> MGSSHHHHHHSQDPNSMTTLTRQDLNFGQVVADVLCEFLEVAVHLILYVREVYPVGIFQKR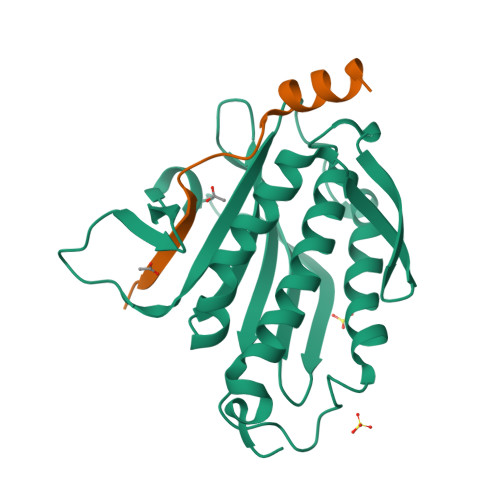KKYNVPVQMSCHPELNQYIQDTLHCVKPLLEKNDVEKVVVVILDKEHRPVEKFVFEITQPPLLSISSDSLLSHVEQLLAAFILKISVCDAVLDHNPPGCTFTVLVHTREAATRNMEKIQVIKDFPWILADEQDVHMHDPRLIPLKTMTSDILKMQLYVEERAHKGS;> MEDKKIVIMPCKCAPSRQLVQVWLQAKE>SMLANSASVRILIKGGKVVNDDCTHEADVYIENGIIQQVGRELMIPGGAKVIDATGKLVIPGGIDTSTHFHQTFMNATCVDDFYHGTKAALVGGTTMIIGHVLPDKETSLVDAYEKCRGLADPKVCCDYALHVGITWWAPKVKAEMETLVREKGVNSFQMFMTYKDLYMLRDSELYQVLHACKDIGAIARVHAENGELVAEGAKEALDLGITGPEGIEISRPEELEAEATHRVITIANRTHCPIYLVNVSSISAGDVIAAAKMQGKVVLAETTTAHATLTGLHYYHQDWSHAAAYVTVPPLRLDTNTSTYLMSLLANDTLNIVASDHRPFTTKQKAMGKEDFTKIPHGVSGVQDRMSVIWERGVVGGKMDENRFVAVTSSNAAKLLNLYPRKGRIIPGADADVVVWDPEATKTISASTQV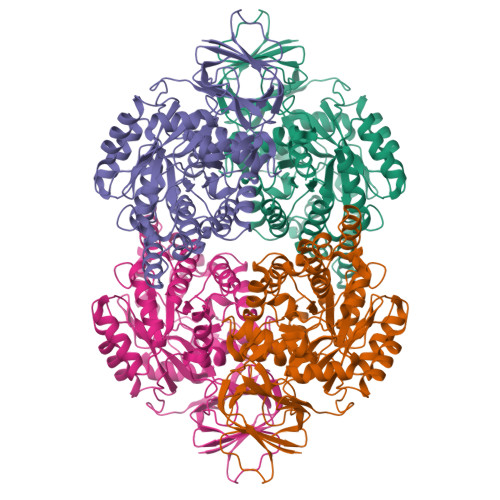QGGDFNLYENMRCHGVPLVTISRGRVVYENGVFMCAEGTGKFCPLRSFPDTVYKKLVQREKTLK[2x]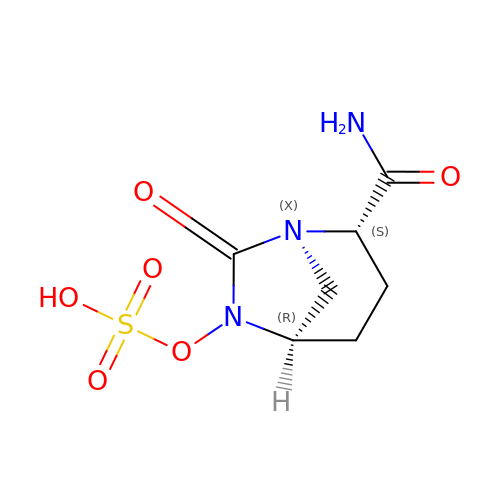(2S,5R)-7-oxo-6-(sulfooxy)-1,6-diazabicyclo[3.2.1]octane-2-carboxamide | C7 H11 N3 O6 S | NDCUAPJVLWFHHB-UHNVWZDZSA-N(2E)-3-{5-[(2,4-diaminopyrimidin-5-yl)methyl]-2,3-dimethoxyphenyl}-1-[(1S)-1-(pentan-3-yl)-3,4-dihydrophthalazin-2(1H)-yl]prop-2-en-1-one 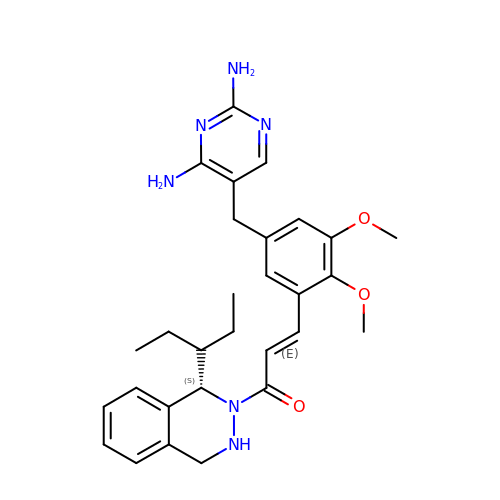| C29 H36 N6 O3 | NVYBVAIPWQNGSG-GIPLCNRYSA-N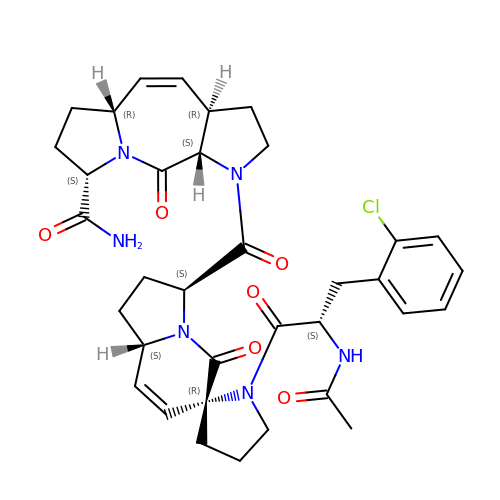(3~{S},7~{R},10~{R},13~{S})-4-[(3~{S},6~{R},8~{a}~{S})-1'-[(2~{S})-2-acetamido-3-(2-chlorophenyl)propanoyl]-5-oxidanylidene-spiro[1,2,3,8~{a}-tetrahydroindolizine-6,2'-pyrrolidine]-3-yl]carbonyl-2-oxidanylidene-1,4-diazatricyclo[8.3.0.0^{3,7}]tridec-8-ene-13-carboxamide | C35 H41 Cl N6 O6 | ITMFJTSTZSWDEK-QHVDBZGRSA-N>MSQHNEKNPHQHQSPLHDSSEAKPGMDSLAPEDGSHRPAAEPTPPGAQPTAPGSLKAPDTRNEKLNSLEDVRKGSENYALTTNQGVRIADDQNSLRAGSRGPTLLEDFILREKITHFDHERIPERIVHARGSAAHGYFQPYKSLSDITKADFLSDPNKITPVFVRFSTVQGGAGSADTVRDIRGFATKFYTEEGIFDLVGHNTPIFFIQDAHKFPDFVHAVKPEPHWAIPQGQSAHDTFWDYVSLQPETLHNVMWAMSDRGIPRSYRTMEGFGIHTFRLINAEGKATFVRFHWKPLAGKASLVWDEAQKLTGRDPDFHRRELWEAIEAGDFPEYELGFQLIPEEDEFKFDFDLLDPTKLIPEELVPVQRVGKMVLNRNPDNFFAENEQAAFHPGHIVPGLDFTNDPLLQGRLFSYTDTQISRLGGPNFHEIPINRPTCPYHNFQRDGMHRMGIDTNPANYEPNSINDNWPRETPPGPKRGGFESYQERVEGNKVRERSPSFGEYYSHPRLFWLSQTPFEQRHIVDGFSFELSKVVRPYIRERVVDQLAHIDLTLAQAVAKNLGIELTDDQLNITPPPDVNGLKKDPSLSLYAIPDGDVKGRVVAILLNDEVRSADLLAILKALKAKGVHAKLLYSRMGEVTADDGTVLPIAATFAG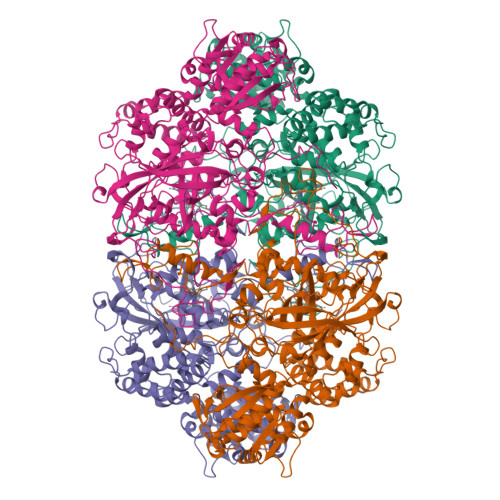APSLTVDAVIVPCGNIADIADNGDANYYLMEAYKHLKPIALAGDARKFKATIKIADQGEEGIVEADSADGSFMDELLTLMAAHRVWSRIPKIDKIPA[4x]>[2x]MINGSKRIAQPIRWAMVGGGRNSQIGYIHRSAALRDQSFALVAGAFDIDPGRGREFGVQLGVDPQRCYPDYRTLFEQEARRPDGIQAVSVATPNGTHFAITRAALEAGLHVVCEKPLCFTLEEAETLREIALANNRVVGVTYGYAGHQLIEQARAMIADGELGEIRMVHMQFAHGFHSAPVEGQNEA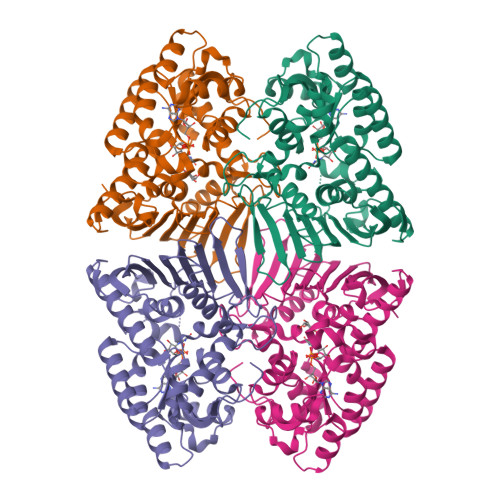TKWRVDPRLAGPSYVLGDVGTHPLYLSEVMLPEFRIKRLMCSRQSFVKSRAPLEDNAYTLMEYEGGAMGLVWSSAVNAGSMHGQKIRVIGSRASLEWWDEHPNQLAFEIQGQPVQVLERGMGYLHPGALLDDRIGAGHPEGLFEAWSNLYYRFAMAMDATERGDGALLAGLRYPDIHAGVEGVRWVERCVQSADRGGVWVDYLAAALEHHHHHH>[4x]QENRLLNESESSSQGLLGYYFSDLNFQAPMVVTSSTTGDLSIPSSELENIPSENQYFQSAIWSGFIKVKKSDEYTFATSADNHVTMWVDDQEVINKASNSNKIRLEKGRLYQIKIQYQREDPTEKGLDFKLYWTDSQNKKEVISSDNLQLPELKQKSSNSLEVLFQGSTSAGPTVPDRDNDGIPDSLEVEGYTVDVKNKRTFLSPWISNIHEKKGLTKYKSSPEKWSTASDPYSDFEKVTGRIDGNVSPEANHPLVAAYPIVHVDMENIILSKNEDQSTQNTDSQTRTISKNTSTSRTHTSEVHGNAEVHASFFDIGGSVSAGFSNSNSSTVAIDHSLSLAGERTWAETMGLNTADTARLNANIRYVNTGTAPIYNVLPTTSLVLGKNQTLATIKAKENQLSQILAPNNYYPSKNLAPIALNAQDDFSSTPITMNYNQFLELEKTKQLRLDTDQVYGNIATYNFENGRVRVDTGSNWSEVLPQIQETTARIIFNGKDLNLVERRIAAVNPSDPLETTKPDMTLKEALKIAFGFNEPNGNLQYQGKDITEFDFNFDQQTSQNIKNQLAELNATNIYTVLDKIKLNAKMNILIRDKRFHYDRNNIAVGADESVVKEAHREVINSSTEGLLLNIDKDIRKILSGYIVEIEDTEGLKEVINDRYDMLNISSLRQDGKTFIDFKKYNDKLPLYISNPNYKVNVYAVTKENTIINPSENGDTSTNGIKKILIFSKKGYEIG;>[4x]QENRLLNESESSSQGLLGYYFSDLNFQAPMVVTSSTTGDLSIPSSELENIPSENQYFQSAIWSGFIKVKKSDEYTFATSADNHVTMWVDDQEVINKASNSNKIRLEKGRLYQIKIQYQRENPTEKGLDFKLYWTDSQNKKEVISSDNLQLPELKQKSSNSLEVLFQGSTSAGPTVPDRDNDGIPDSLEVEGYTVDVKNKRTFLSPWISNIHEKKGLTKYKSSPEKWSTASDPYSDFEKVTGRIDKNVSPEARHPLVAAYPIVHVDMENIILSKNEDQSTQNTDSQTRTISKNTSTSRTHTSEVHGNAEVHASFFDIGGSVSAGFSNSNSSTVAIDHSLSLAGERTWAETMGLNTADTARLNANIRYVNTGTAPIYNVLPTTSLVLGKNQTLATIKAKENQLSQILAPNNYYPSKNLAPIALNAQDDFSSTPITMNYNQFLELEKTKQLRLDTDQVYGNIATYNFENGRVRVDTGSNWSEVLPQIQETTARIIFNGKDLNLVERRIAAVNPSKPLETTKPDMTLKEALKIAFGFNEPNGNLQYQGKDITEFDFNFDQQTSQNIKNQLAELNATNIYTVLDKIKLN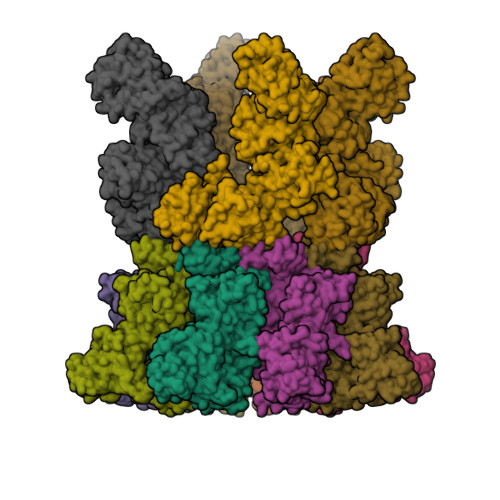AKMNILIRDKRFHYDRNNIAVGADESVVKEAHREVINSSTEGLLLNIDKDIRKILSGYIVEIEDTEGLKEVINDRYDMLNISSLRQDGKTFIDFKKYNDKLPLYISNPNYKVNVYAVTKENTIINPSENGDTSTNGIKKILIFSKKGYEIG;>MNEHYTESDIKRNHKTEKNKTEKEKFKDSINNLVKTEFTNETLDKIQQTQDLLKKIPKDVLEIYSELGGEIYFTDIDLVEHKELQDLSEEEKNSMNSRGEKVPFASRFVFEKKRETPKLIINIKDYAINSEQSKEVYYEIGKGISLDIISKDKSLDPEFLNLIKSLSDDSDSSDLLFSQKFKEKLELNNKSIDINFIKENLTEFQHAFSLAFSYYFAPDHRTVLELYAPDMFEYMNKLEKGGFEKISESLKKEGVEKDRIDVLKGEKALKASGLVPEHADAFKKIARELNTYILFRPVNKLATNLIKSGVATKGLNVHGKSSDWGPVAGYIPFDQDLSKKHGQQLAVEKGNLENKKSITEHEGEIGKIPLKLDHLRIEELKENGIILKGKKEIDNGKKYYLLESNNQVYEFRISDENNEVQYKTKEGKITVLGEKFNWRNIEVMAKNVEGVLKPLTADYDLFALAPSLTEIKKQIPQKEWDKVVNTPNSLEKQKGVTNLLIKYGIERKPDSTKGTLSNWQKQMLDRLNEAVKYTGYTGGDVVNHGTEQDNEEFPEKDNEIFIINPEGEFILTKNWEMTGRFIEKNITGKDYLYYFNRSYNKIAPGNKAYIEWTDPITKAKINTIPTSAEFIKNLSSIRRSSNVGVYKDSGDKDEFAKKESVKKIAGYLSDYYNSANHIFSQEKKRKISIFRGIQAYNEIENVLKSKQIAPEYKNYFQYLKERITNQVQLLLTHQKSNIEFKLLYKQLNFTENETDNFEVFQKIIDEK[4x]> GPLGSMFERFTDRARRVVV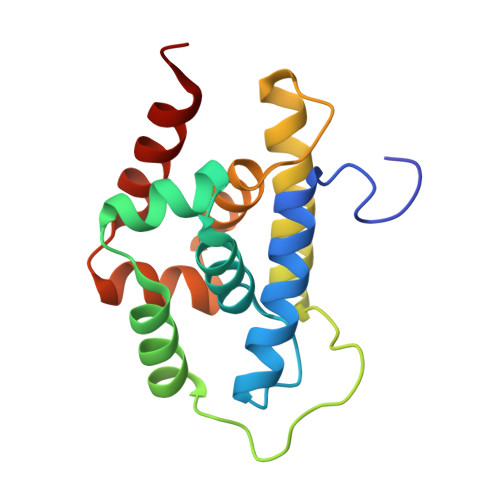LAQEEARMLNHNYIGTEHILLGLIHEGEGVAAKSLESLGISLEGVRSQVEEIIGQGQQAPSGHIPFTPRAKKVLELSLREALQLGHNYIGTEHILLGLIREGEGVAAQVLVKLGAELTRVRQQVIQLLSGY>[8x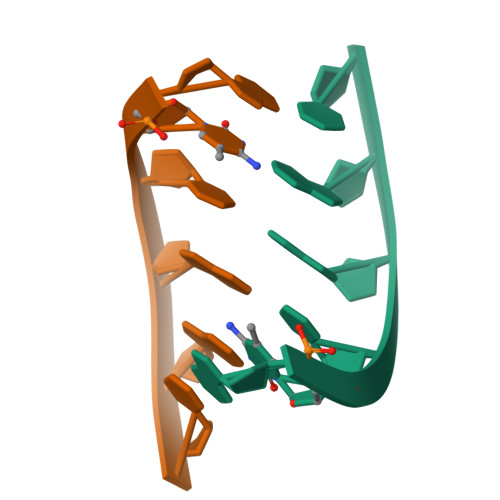]GCTAGC>GSMTDSEKSATIKVTDASFATDVLSSNKPVLVDFWATWCGPSKMVAPVLEEIATERATDLTVAKLDVDTNPETARNFQVVSIPTLILFKDGQPVKRIVGAKGKAA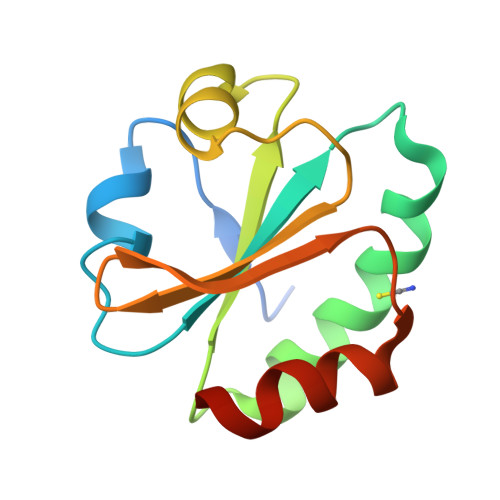LLRELSDVVPNLN[2x]> MASVSAGESVQITLPKNEVQLNAYVLQEPPKGETYTYDWQLITHPRDYSGEMEGKHSQILKLSKLTPGLYEFKVIVEGQNAHGEGYVNVTVKPEPRKNRPPIAIVSPQFQEISLPTTSTVIDGSQSTDDDKIVQYHWEELKGPLREEKISEDTAILKLSKLVPGNYTFSLTVVDSDGATNSTTANLTVNKAVDYPPVANAGPNQVITLPQNSITLFGNQSTD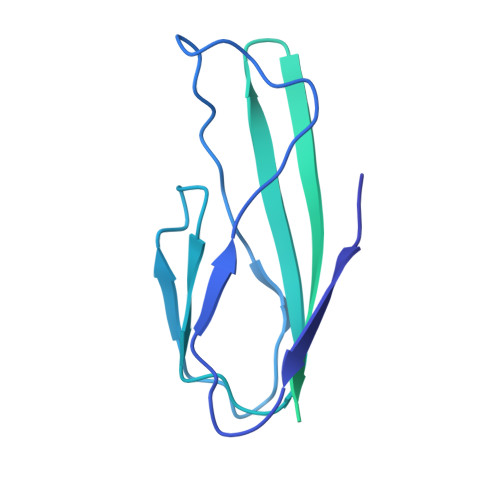DHGITSYEWSLSPSSKGKVVEMQGVRTPTLQLSAMQEGDYTYQLTVTDTIGQQATAQVTVIVQPENNK>ALTSNASGTFDGYYYELWKDTGNTTMTVYTQGRFSCQWSNINNALFRTGKKYNQNWQSLGTIRITYSATYNPNGNSYLCIYGWSTNPLVEFYIVESWGNWRPPGATSLGQVTIDGGTYDIYRTTRVNQPSIVGTAT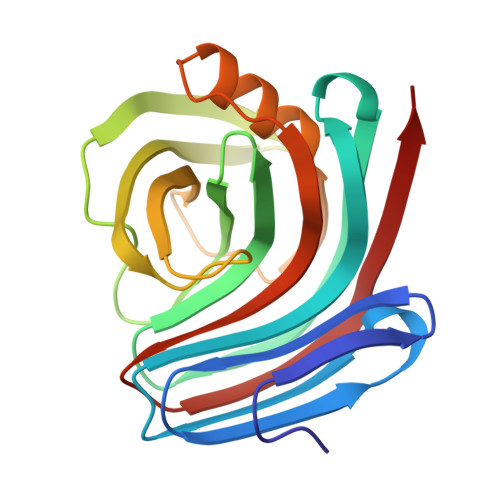FDQYWSVRTSKRTSGTVTVTDHFRAWANRGLNLGTIDQITLCVEGYQSSGSANITQNTFSQSS[2x]> GYEREDDGVPS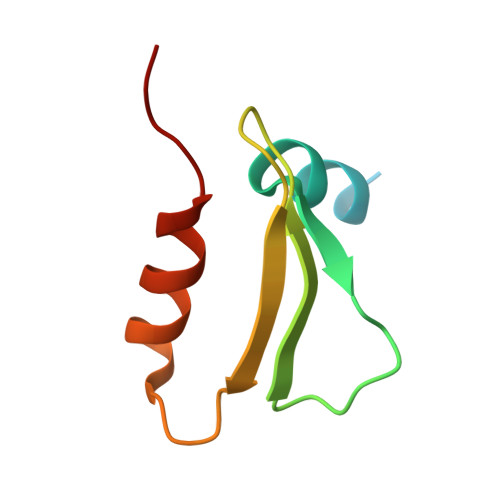AAYVTQLYYKISRIDWDYEVEPARIKGIHYGPDIAQPINMDSSHHSRCFISDYLWSLVPTAW>[2x]ALTPMEFARKYNLLRKDDALL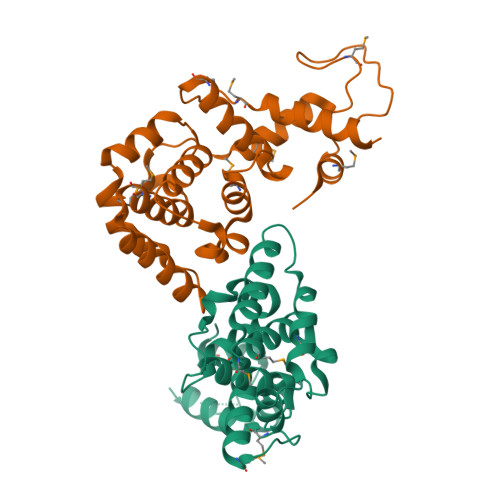DNPVPGEEMTAGIRRGDAKRVFTMQLGPYWDGFERCSPQAYALSAVFMARMNRDRDAANNILKVLDKTFVDGKPDFSVARPVMKKYQNSELVQEVVAKHAYVLTVIASLLEAAREDGVVPSSEFLWLKPVDRRLWYMLNCVGRQTPYSEVAGPFAHWKAEKEMGRRSLVPMIDEAIRALEIAVKEVR> ANGNEGLSTTTKYIFVPIATIGCGKTTVF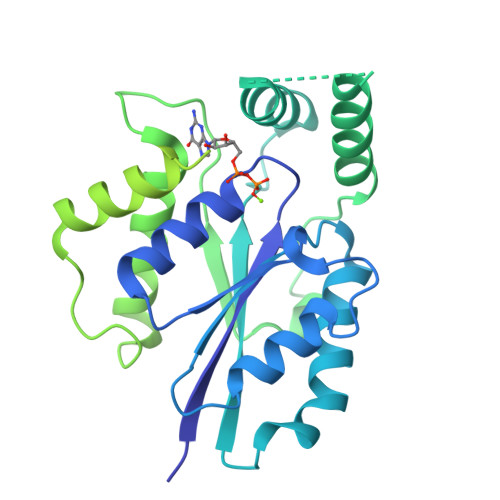NTLNNLFPQWTHIQNDNISKKAKLKICDLTLLALEDDDQSVVLFDRNNSASRERRQIFTTIDQKRDEHLDDTVDLKYIAINFIPEDLSEEELWDITYNRVIQRGDNHQSIKSQLDENLVESVMKGFIQRYQPINTSRSPDDQFDHVIHLKLSKDENSLKSSLENVRIIIDDLVQNFPDLIKEKPADELINECFQKALDYKPTFVKNMTANTIKKDPTYYGIAMHYSSILENLEIVSHNEHFQNIKSHIQTEFHVTLGHIASSKQDKAGRVKWKKLVKTLGKGDPNKPKSALKFFADVKLLQIVINTDKLACIKVEILKIYDTNDVLQSEIEPINKQLHITIGCIPPATAVESNITLEELYDNPDEQELKPDGTYKCGDDTLHVFNFDNPDLKLFSQQLFVAYQPTFVKN>[2x]MKHHHHHHDEIISELRELCLNYIEQDERLSRQKLNFLGQREPRMVLIEGLKLLSRCIEIDSADKSGCTHNHDDKSVETILVESGIVCPGLPLIIPDGYKLI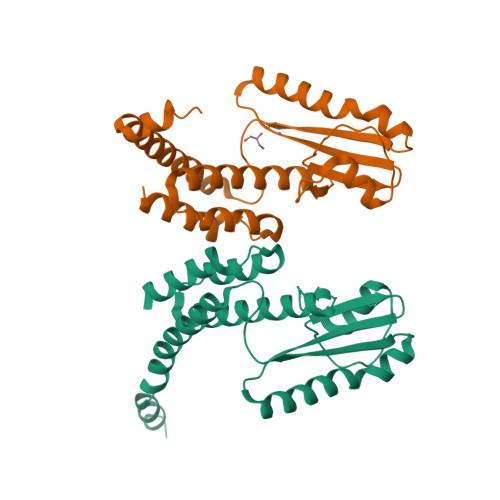DNSLILLECFVRSTPASFEKKFIEATNKLACIREDLAVAGVTLVPIVDGRCDYDNSFMPEWANFKFRDLLFKLLEYSNQDEKVFEESEYFRLCESLKTTIDKR>[3x]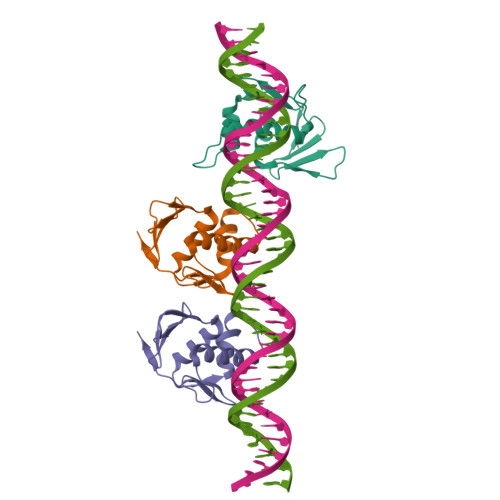MKFILAEKFTFDPLSNTLIDKEDSEEIIRLGSNESRILWLLAQRPNEVISRNDLHDFVWREQGFEVDDSSLTQAISTLRKMLKDSTKSPQYVKTVPKRGYQLIARVETV>[2x]DSAAYQRTSLYGDDVVIVAAHRTPLCKSKRGNFKDTYPDDLLAPVLRALIEKTNLNPSEVGDIVVGTVLAPGSQRASECRMAAFYAGFPETVAVRTVNRQCSSGLQAVADVAAAIKAGFYDIGIGAGLESMTTNPMAWEGSVNPAVKKFAQAQNCLLPMGVTSENVAQRFGVSRQEQDQAAVDSHRKAAAATAAGKFKDEIIPVKTKLVDPKTGDEKPITVSVDDG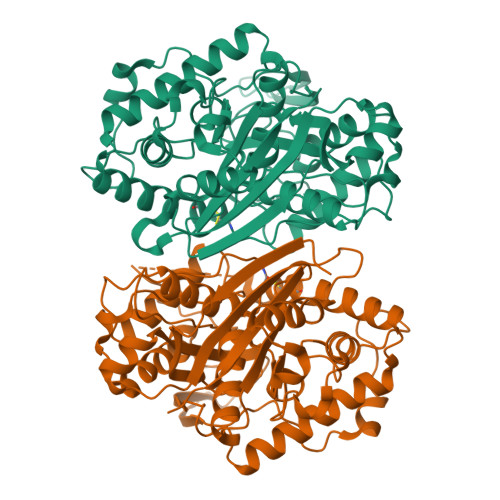IRPTTTLASLGKLKPVFKKDGTTTAGNSSQVSDGAGAVLLMKRSVAMQKGLPVLGVFRTFAAVGVDPAIMGIGPAVAIPAAVKAAGLELDDIDLFEINEAFASQFVYCRNKLGLDPEKINVNGGAMAIGHPLGATGARCVATLLHEMKRRGKDCRFGVVSMCIGTGMGAAAVFERGDG> MMSREALQETLSAVMDNEADELELRRVLAACGEDAELRSTWSRYQLARS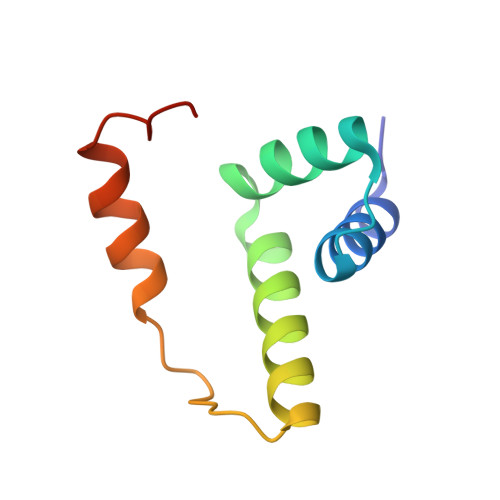VMHREPTLPKLDIAAAVSAALADEAAPPKAEK[(2~{R},3~{R},4~{R},5~{S})-5-(6-aminopurin-9-yl)-3,4-bis(oxidanyl)oxolan-2-yl]methyl [(2~{R},3~{R},4~{S},5~{R})-2-(2-azanyl-6-oxidanylidene-1~{H}-purin-9-yl)-5-(hydroxymethyl)-4-oxidanyl-oxolan-3-yl] 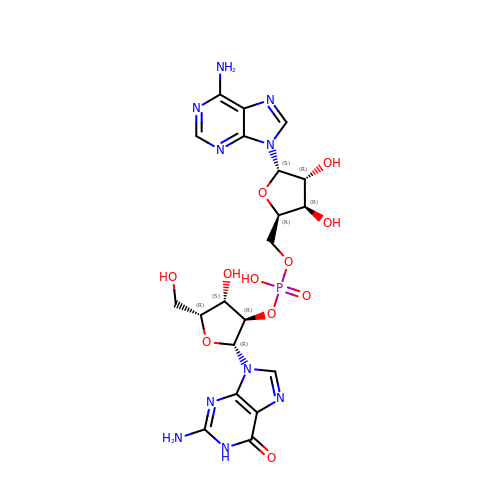hydrogen phosphate | C20 H25 N10 O11 P | ZLNKIMYMVZHDPX-UHFFFAOYSA-N> ANLYFQSDREEFQWLVEEFIRVLERGDVEKAREILRLLKEVAEKVNDPLLRLL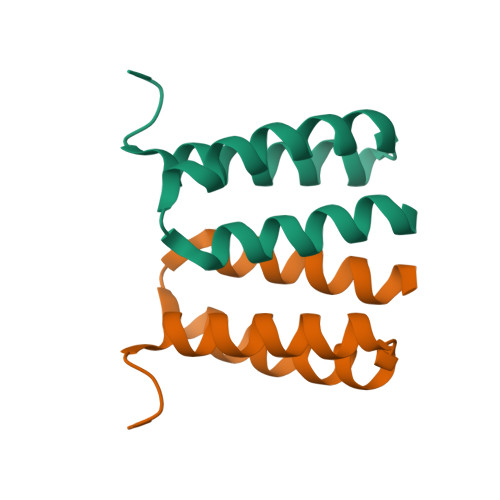FRIARRLVEEL> GSHMASSGKKFYAKFGQRSARCNYKIQLDSNKIVDTVDIEDIGEKKAFCRCWKSE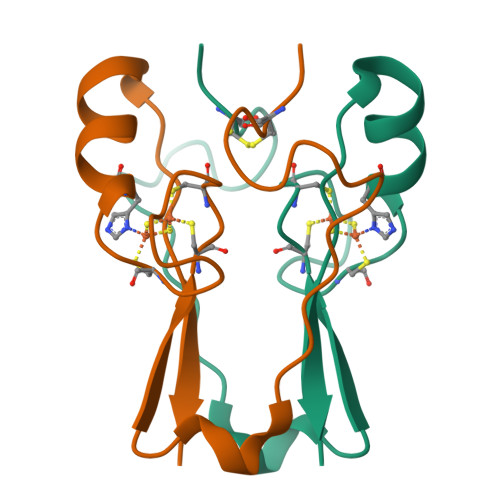KWPYCDGSHGKHNKETGDNVGPLIVKSEKK>[2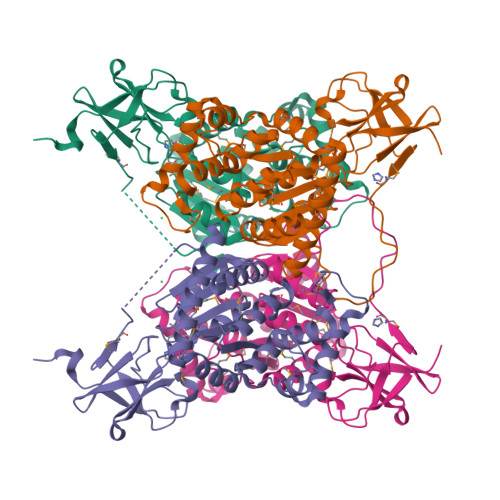x]SNANIPEIENANLKPALKDSVLPDGFYSTTNHPTHVKVNDEWIEVANPKMDAVIVVYPEEKRAETKVIRKVKKGDFVLIGHNGIRVMPPEKSREAGQLFEFMNSEVSSEKPKEAIIKRIAKEMHEIREEYKKTGTGGIAIVGGPAIIHTGGGPALAKMVELGYIQAILAGNALATHDIESALYGTSLGVNIKTAKPVTGGHKHHIYAINAINDAGNIKNAVESGVLKEGIMYQCIKNNIPYVLAGSIRDDGPIPDVITDSMVAQDKMRTTVMDKKMVIMLSTLLHSVATGNLMPSYIKTVCVDIQPSTVTKLMDRGTSQAIGVVTDVGVFLVLLLKELERLELQE> MFRRIAGFSPIFLMLFGSSLPTMGNPVKREIHPDAVFYKEHKLRNDGLVITTNQGNIRLQFKSEAAIEVLYRADSKQLPSFALAQPESAIKAQLTETENHLQFSGGTLTARIQKRPFAISYYRDSELLLAEESGFQVNTDKINFRFYLSPGEKILGGGQRILGMDRRGQRFPLYNRAHYGYSDHSGQMYFGLPAIMSSKQYILVFDNSASGAMDIGKTESDILQLEAKSGRS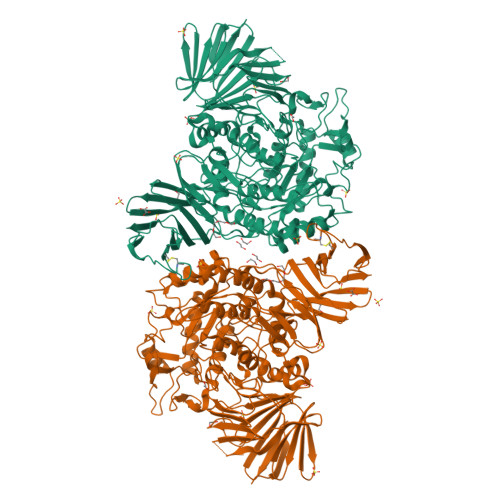AYILVAGNSYPSLIENFTQVTGRQPLPPRWALGSFASRFGYRSEAETRATVQKYKTEDFPLDTIVLDLYWFGKDIKGHMGNLDWDKENFPTPLDMMADFKQQGVKTVLITEPFVLTSSKRWDDAVKAKALAKDPQGQPKAFELYFGNGGIIDVFSKEGSRWFSSIYKDLSKQGVAGWWGDLGEPEMHPEDTQHAIGDADTVHNAYGHRWAEMLYQQQLDQFPELRPFIMMRAGFVGSQRYGMIPWTGDVSRTWGGLASQVELALQMSLLGFGYIHSDLGGFADGETLDKEMYIRWLQYGVFQPVYRPHGQDHIPSEPVFQDEETKAILRPLVKLRYRMLPYIYTAAYQNTLTGMPLMRPLFFSDEKNPALIDNKTSYFWGDSLLVTPITQAGVESVSIPAPKGVWFDFWKDTRYQTDGAPLTLPTDLHTIPVLVKAGAFMPYVPAVSTTEDYRSDSLEIHYYADASVPLAQGEIFEDDGKDPNSIKRNQFDLLTLQATHTDNQLHFQLARTGKGYRGMPERRATTLVIHNASDQYQHLDINGKTIAIAQADCASTPALACYDQERRQLQLVFTWGREALNLRLHK>MSSYSNKDVQRGDASMHHYQWAKTPPMGWNSWDCYGASVTEDEVKGNAEYMAKYLKPFGWEYVVVDIQWYEPGANSSIYRPFVPLEMDEYSRLMPAVNRFPSAKGGKGFKPLADYIHNLGLKFGIHIMRGIPRQAVHQNTPILGTNVGARDIADTNSICPWNTDMYGVDHRKEGAQAYYDSLFQLYAQWGVDFVKVDDIVASKLYGTHTEEIKMIRKAIDRCGRPIVLSLSPGPAPLDHATLFVENANMWRMTDDFWDRWELLYDMFEQCYKWCKLVGLGHWPDADMLPLGHIGIRSVDGGG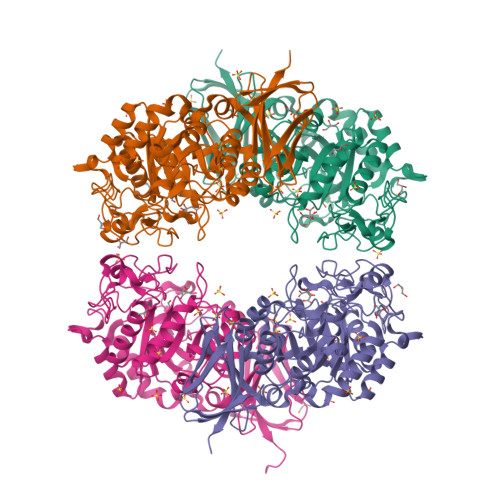TDRMTRFTKDEQRTMMTLWIIFRSPLMFGGELRDNDEWTLSLLTNEEVLHVHQNGYGARQVYRENDHVVWTSQDAEGNQFVAMFNISEKRSVVSVSLKDLGCMEPMKARDLWAKEDLGLVKHQLAFELGPHQSILVKLSPAVGKGL[8x]KAI2 receptors, classified as plant α/β hydrolase enzymes, are capable of perceiving smoke-derived butenolide signals and endogenous yet unidentified KAI2-ligands (KLs). The KAI2-mediated signaling pathway shows homology to another phytohormone signaling pathway, strigolactone (SL), where key proteins involved in KAR signaling (KAI2, D3/MAX2, and SMAX1/2) share sequence and structural similarities with proteins in the SL signaling pathway. The SL signaling pathway comprises a homologous receptor to KAI2, D14 (DWARF14), the D3/MAX2 E3 ligase, and a homologous substrate SMAX1-LIKE 6, 7, and 8 (SMXL) in Arabidopsis or D53 (DWARF53) in rice. When focusing on the binding pocket, several residues including the Ser-His-Asp catalytic triad are conserved in all proteins, highlighting its importance in the catalytic mode of action performed by α/β hydrolases.

The OsKAI2 and AtKAI2 structures were also compared to the analogous receptors for SL signaling in both rice OsD14 (49), and in the model plant Arabidopsis, AtD14. To that end, we determined a new AtD14 crystal structure at a higher resolution (2 Å) than the previously reported structures and was hence applied here for comparative analysis. Structural superposition with OsKAI2 showed an RMSD of 1.2 Å over 265 Cα and 1.2 Å over 264 Cα for OsD14 and AtD14 respectively, and both D14s gave a sequence identity of 56%, confirming high structural similarity in all four proteins examined here. However, there are some clear differences in both the positioning and type of residue found in the pocket when comparing the KAI2s and D14s. Most noticeably, F27/F26 in OsKAI2 and AtKAI2 are shifted by 1.2 Å in respect to the positioning of F28 in both D14s. Similarly, F195 in both KAI2s is shifted into the pocket by 2.7 Å when compared to F195 in both D14s. Furthermore, both KAI2s possess Y125/124 in place of F126 in D14s, with the hydroxyl group reaching 1.3 Å further into the pocket; similarly, both KAI2s possess the larger hydrophobic I194 in place of V194 seen in the D14s. Conversely, we found that A220 in both rice and Arabidopsis KAI2s is replaced with S220 in D14s which is slightly larger and more polar, perhaps indicating a role in strigolactone binding. Collectively, the differences between KAI2 and D14s demonstrate that distinct residues reach further into the pocket in the KAI2s, suggesting an adapted and more compact pocket to better fit KL/SL-like ligands. Generally, SL receptor D14 responds to (+)-GR24 due to its similarity to natural SLs, whilst KAI2 proteins tend to respond to (−)-GR24 more readily.

>[2x]MSQHNILEALNVRVVGTGDRILFLAHGFGTDQSAWHLILPYFTQNYRVVLYDLVCAGSVNPDYFDFNRYTTLDPYVDDLLNIVDSLGIQNCAYVGHSVSAMIGIIASIRRPELFSKLILIGFSPRFLNDEDYHGGFEEGEIEKVFSAMEANYEAWVHGFAPLAVGADVPAAVREFSRTLFNMRPDISLFVSRTVFNSDLRGVLGLVRVPTCVIQTAKDVSVPASVAEYLRSHLGGDTTVETLKTEGHLPQLSAPAQLAQFLRRALPR>MNHKVHHHHHHIEGRHMQILSPENAPRIGFIGFGAMASRMGDHLKTAGYTISAYTPSGRSPSPSVPMLPTPLALAKQADTVVVCVPDDEALAASMYGENGALAGMTKGSLLINTSSVS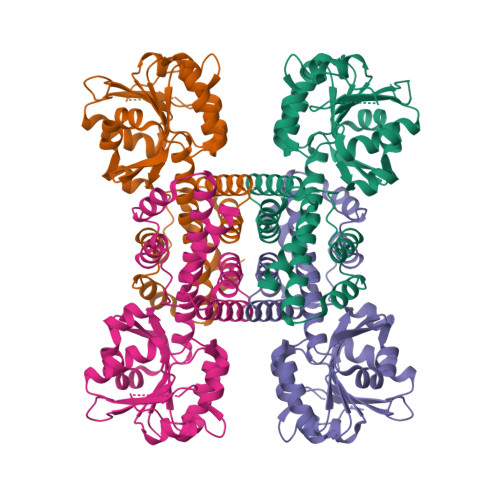PEATATLYEAGQKHGVVVLDAPVSGSTPEADSASLVILVGGDKDDVARAAPIFDAIGKLTIHAGPTGSGARLKLVINGIMGAGLTTLAESVAYGLSAGLDRSMLFDALDQVAVISPHHKRKLKAAKDGNFAPQFPARLMQKDMRLLLDAAAREAVPVPTLAAATQQLSLTRRLSPNEDYSSLIRVMEKIVANDRY[8x]>[2x]HHHHHHMATETNYPVPYRSKLTEPFEPGQTLIIKGKTAEDSVRFTINLHNTSADFSGNDVPLHISVRFDEGKIVFNTFSKGEWGKEERKSNPYKKGDDIDIRIRAHDSKFSISVDQKEVKEYEHRVPLSSVTHFSVDGDILITY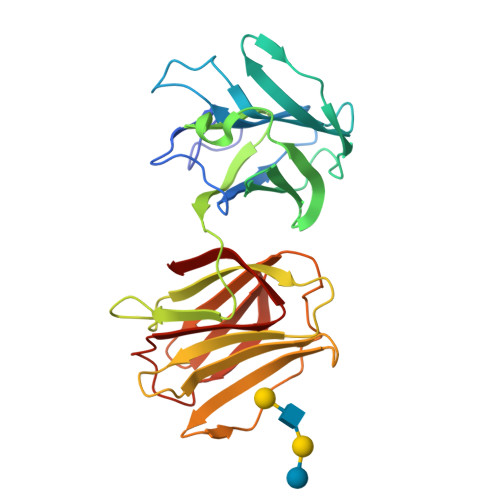IHWGGKYYPVPYESGLAGDGLAPGKSLLIFATPEKKGKRFHINLLKKNGDIALHFNPRFDEKAIVRNSLISGEWGNEEREGKNPLEKGIGCDLEFRNEEYAFQIYVDGERFATYAHRLDPHDINGLQIGGDVEVTGIQMV>[2x]SELSFNYPNFQSVEDITFQGGASPRNETLQLTPTDSNGIPIRQRAGHAVYSQPFQLRDTSFYTTFTFVIRTTSNSPADGF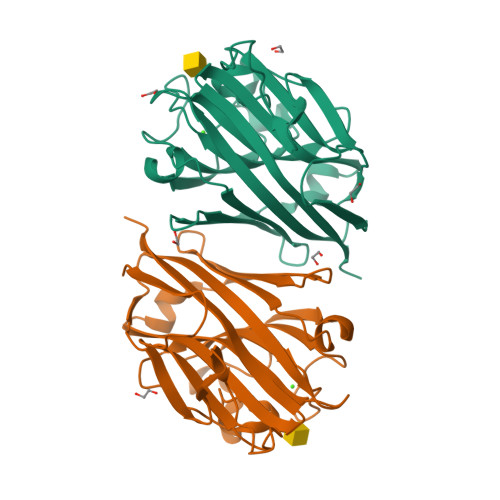AIFIAPPDFPVKRYGGYLGLFEPNTATNTSANKVVAVEFDTWVNTEWKEPRYRHIGIDVNSIVSVRVTRWQDKDVFSRSIATAHVGYDGISKILTAFVTYPDGGNYVLSHVVDLAEIFPGDVRIGFSGATGQYETQYIHSWSFSSTSTNLLRDGARHHHHHH> MGHHHHHHLESTSLYKKSSSTPPRGVTVVNNFDCKRYLGTWYEIARFDHRAERGLEKVTATYSLRDDGGLNVIFKGYNPDRGMWQQYVGKAYF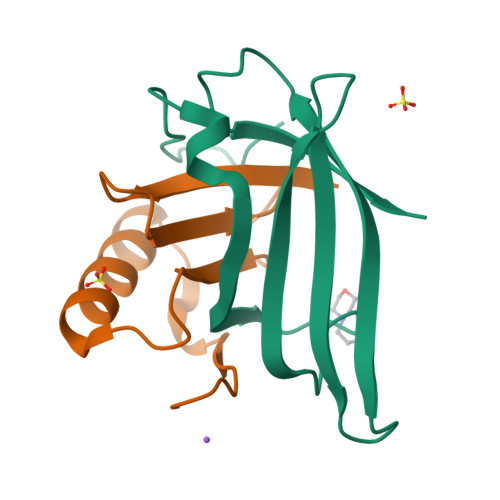TGAPTRAALKVAFF;> MGPFYGGYNVIALDREYRHALVCGPDRDYLWINSRTPTISDEVKQEMLAVATREGFDVSKFIWVQQPGS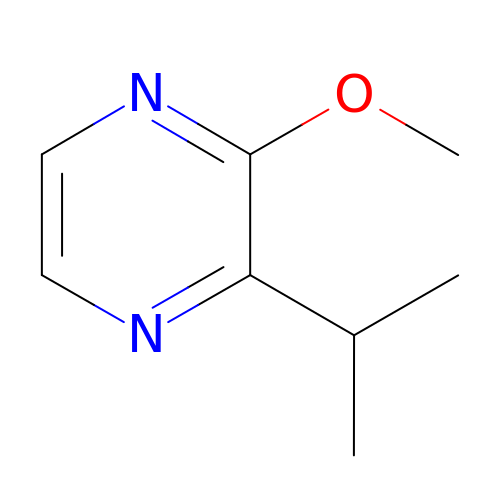2-ISOPROPYL-3-METHOXYPYRAZINE | C8 H12 N2 O | NTOPKICPEQUPPH-UHFFFAOYSA-N> MSADAQSFLNRVCGVSAARLTPCGTGTSTDVVYRAFDIYNDKVAGFAKFLKTNCCRFQEKDEDDNLIDSYFVVKRHTFSNYQHEETIYNLLKDCPAVAKHDFFKFRIDGDMVPHISRQRLTKYTMADLVYALRHFDEGNCDTLKEILVTYNCCDDDYFNKKDWYDFVENPDILRVYANLGERVRQALLKTVQFCDAMRNAGIVGVLTLDNQDLNGNWYDFGDFIQTTPGSGVPVVDSYYSLLMPILTLTRALTAESHVDTDLTKPYIKWDLLKYDFTEERLKLFDRYFKYWDQTYHPNCVNCLDDRCILHCANFNVLFSTVFPPTSFGPLVRKIFVDGVPFVVSTGYHFRELGVVHNQDVNLHSSRLSFKELLVYAADPAMHAASGNLLLDKRTTCFSVAALTNNVAFQTVKPGNFNKDFYDFAVSKGFFKEGSSVELKHFFFAQDGNAAISDYDYYRYNLPTMCDIRQLLFVVEVVDKYFDCYDGGCINANQVIVNNLDKSAGFPFNKWGKARLYYDSMSYEDQDALFAYTKRNVIPTITQMNLKYAISAKNRARTVAGVSICSTMTNRQFHQKLLKSIAATRGATVVIGTSKFYGGWHNMLKTVYSDVENPHLMGWDYPKCDRAMPNMLRIMASLVLARKHTTCCSLSHRFYRLANECAQVLSEMVMCGGSLYVKPGGTSSGDATTAYANSVFNICQAVTANVNALLSTDGNKIADKYVRNLQHRLYECLYRNRDVDTDFVNEFYAYLRKHFSMMILSDDAVVCFNSTYASQGLVASIKNFKSVLYYQNNVFMSEAKCWTETDLTKGPHEFCSQHTMLV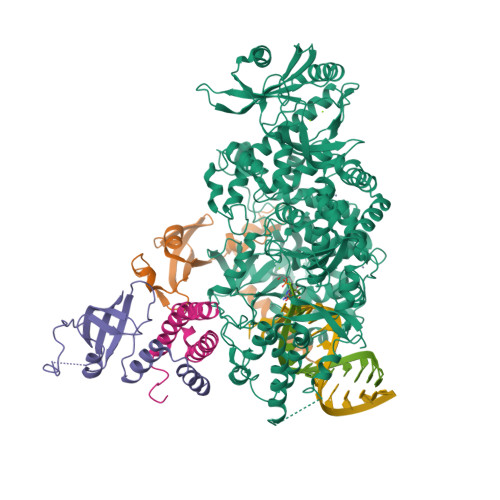KQGDDYVYLPYPDPSRILGAGCFVDDIVKTDGTLMIERFVSLAIDAYPLTKHPNQEYADVFHLYLQYIRKLHDELTGHMLDMYSVMLTNDNTSRYWEPEFYEAMYTPHTVLQGGSENLYFQG;>[2x]MAIASEFSSLPSYAAFATAQEAYEQAVANGDSEVVLKKLKKSLNVAKSEFDRDAAMQRKLEKMADQAMTQMYKQARSEDKRAKVTSAMQTMLFTMLRKLDNDALNNIINNARDGCVPLNIIPLTTAAKLMVVIPDYNTYKNTCDGTTFTYASALWEIQQVVDADSKIVQLSEISMDNSPNLAWPLIVTALRANSAVKLQ;> MSKMSDVKCTSVVLLSVLQQLRVESSSKLWAQCVQLHNDILLAKDTTEAFEKMVSLLSVLLSMQGAVDINKLCEEMLDNRATLQ> MANTKYNKEFLLYLAGFVDGDGSIIAQINPNQSSKFKHRLRLTFYVTQKTQRRWFLDKLVDEIGVGYVRDSGSVSQYVLSEIKPLHNFLTQLQPFLKLKQKQANLVLKIIEQLPSAKESPDKFLEVCTWVDQIAALNDSKTRKTTSET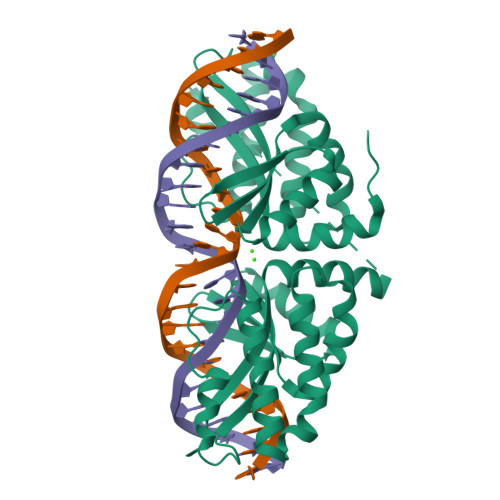VRAVLDSLSGKKKSSPAAGGSDKYNQALSKYNQALSKYNQALSGGGGSNKEFLLYLAGFVDSDGSIIAQIKPRQSNKFKHQLSLTFAVTQKTQRRWFLDKLVDEIGVGYVYDSGSVSDYRLSEIKPLHNFLTQLQPFLKLKQKQANLVLKIIEQLPSAKESPDKFLEVCTWVDQIAALNDSKTRKTTSETVRAVLDSLSEKKKSSPLEHHHHHH> LFPGCARRPVAPLAHAMSPSVLVPAGLAGIQDGRGRFREIMTAIMADHGAFLPGDRSSDGDGILWRLAGEPGPTGRPVPLGVSTAGIRLVLVPGLLAECVSESSLLFDDARPDVERYGYATTLVRTGGRWGSARNAAIIHEVVAKLPENDTIVFVTHSKGAVDVLEALVSYPDLAARTAAVVSVAGAIDGSPLAETFS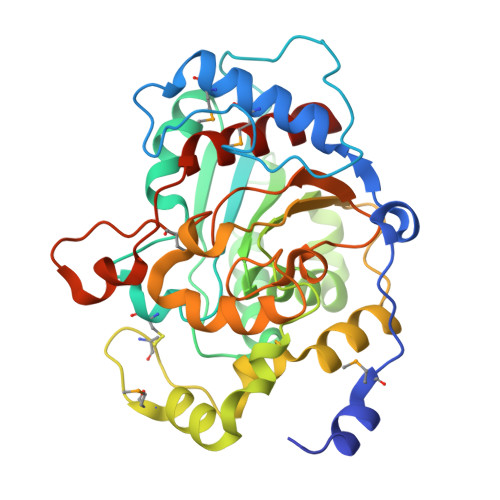DGLLRFAESMPLSSCPPGEGTEALDSLKRAYRLRFLAEHRLPARVRYYSLAAFASREETSAILRPFYDILAKTDALNDGLVIAADAIIPGGTLLGYPNADHLAVAMPFSKKPSLLTSVISKNSYPRPALLEAIARYVEEDLGPEKGREN> MGSSHHHHHHSSGLVPRGSNFAYLNTQSNHDKQYIGHAGELRVLSQRIAKNATEAAAGKGEAFKLLKDARNDFEKRWNILVNGDESTSLPPSPEAVKPQMDVVQQDWDGLRKNADSILASEQTVLSLHQVASTLAETIPQLQVEYEEVVDILLENGAPADQVAVAQRQSLLAERILGSVNKVLAGDE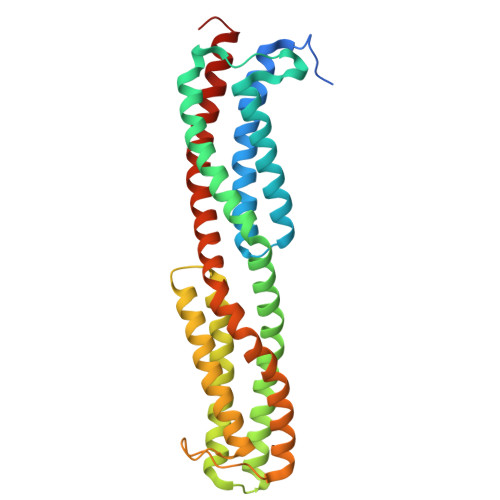NSVQAADSFGRDASLFGRVLKGMQEGNAAMSISKVTNAEAVDRLNEIAELFEFVSGSVDEILETSPDLFQVREAANNIFSVSQTLLDKASQLADGFENLAGGRSIN>GMKTIIRQPQLYRFLKYCNESNLDKTVLDCGAGGDLPPLSIFVEDGYKTYGIEISDLQLKKAENFSRENNFKLNISKGDIRK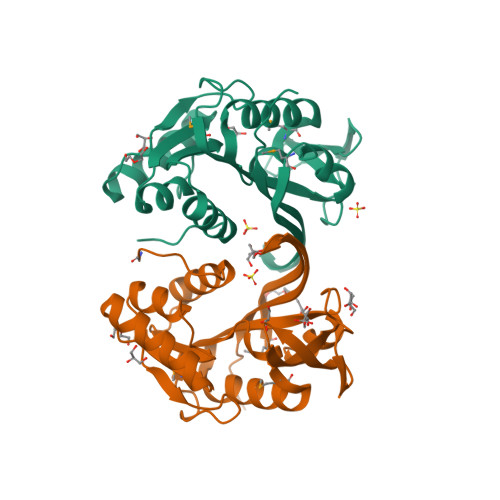LPFKDESMSFVYSYGTIFHMRKNDVKEAIDEIKRVLKPGGLACINFLTTKDERYNKGEKIGEGEFLQLERGEKVIHSYVSLEEADKYFKDMKVLFKEDRVVERINDGLKIKQGYVDYIAEKFSKSIL[2x]> MSWATRLLRMSSPRLGLLPLGRSVKLGGAKERVSFSQFF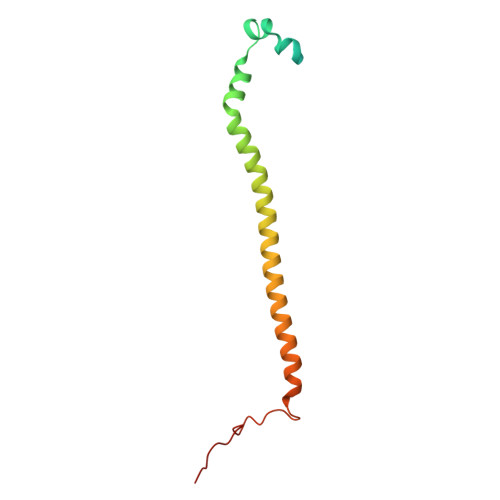DSEYFWTKANVGPFFLFLFTSPFWYQGIKTVYASCRYRKLNEREIISDRYTWLHERMLEDEVERVLLEQVPAGGFDKTRPGLLLGPSTL>GSVRIPVSCRHSGQCLRPCRDAGMRFGRCMNGRCDCTPR[2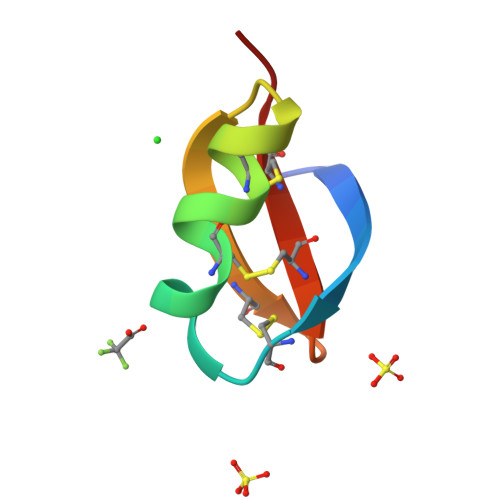x]Volume-regulated anion channels (VRACs) constitute a diverse family of ion channels that are ubiquitously expressed in mammalian cells. They are believed to be essential for maintaining cellular volume, as they are known to open in response to hypotonic stress, enabling efflux of anions and osmolytes, thereby preventing excessive cell swelling and burst. VRACs are hexamers composed of five closely related paralogues of the leucine-rich repeat-containing protein 8 family (termed LRRC8A to E). In contrast, when expressed on its own, the LRRC8C subunit forms a larger, heptameric assembly with weaker mutual subunit interactions and a different preferential arrangement of the LRRDs.

In the framework of a large-scale, exome-based genetic analysis of patients with rare undiagnosed disorders, we identified a 1-bp heterozygous insertion in the gene LRRC8C in an Italian boy (P1) presenting with marked skin telangiectasia and gastrointestinal vascular dysplasia, microcephaly, intellectual disability, skeletal dysplasia with fragile bones, and eye abnormalities including optic atrophy. This DNA variant, NM_032270.4:c.1197dup, p.(Leu400IlefsTer8) (NC_000001.11:g.89713767dup [hg38], NC_000001.10:g.90179326dup [hg19]), produced a shift of the reading frame leading to the change of Leu 400 to Ile and the insertion of six amino acids followed by a premature termination codon. Like most variant-induced interruptions of the coding frame located in the last exon of a gene, c.1197dup (from now on, ‘LRRC8Ctrunc’) is predicted to escape nonsense-mediated mRNA decay and result in the production of a truncated protein product. In the case of LRRC8Ctrunc, we found a similar behavior as for full-length subunits, with a monodisperse peak eluting at somewhat larger volume, which is consistent with the smaller size of a channel that lacks its LRRDs. In independent datasets of each mutant, we found an equivalent heptameric organization as for WT, but also distinct differences in the observed structural features (Table EV1). In both cases, this is manifested in weak density for large parts of the protein, which likely reflects an increased molecular mobility as a consequence of altered subunit interactions. The differences are particularly evident for LRRC8Ctrunc, where the extracellular part of the pore domain carrying the narrow selectivity filter is well-defined as structural unit obeying C7 symmetry. Whereas the extracellular sub-domain (ESD) closely resembles the equivalent region of WT, parts of the protein located further in intracellular direction are not resolved in the density as a consequence of their structural heterogeneity.

>MSIPVTEFRQFSEQQPAFRVLKPWWDVFTDYLSVAMLMIGVFGCTLQVMQDKIICLPKRVQPAQNHSSLSNVSQAVASTTPLPPPKPSPANPITVEMKGLKTDLDLQQYSFINQMCYERALHWYAKYFPYLVLIHTLVFMLCSNFWFKFPGSSSKIEHFISILGKCFDSPWTTRALSEVSGEDSEEKDNRKNNMNRSNTIQSGPEGSLVNSQSLKSIPEKFVVDKSTAGALDKKEGEQAKALFEKVKKFRLHVEEGDILYAMYVRQTVLKVIKFLIIIAYNSALVSKVQFTVDCNVDIQDMTGYKNFSCNHTMAHLFSKLSFCYLCFVSIYGLTCLYTLYWLFYRSLREYSFEYVRQETGIDDIPDVKNDFAFMLHMIDQYDPLYSKRFAVFLSEVSENKIKAAELKALEVLFQ[7x]> IESIIKTATDTVKSEINAELGVVPSLNAVETGATSNTEPEEAIQTRTVINQHGVSETLVENFLSRAALVSKRSFEYKDHTSSAAQTDKNFFKWTINTRSFVQLRRKLELFTYLRFDAEITILTTVAVNGSSNNTYMGLPNLTLQAMFVPTGALTPEKQDSFHWQSGSNASVFFKISDPPARMTIPFMCINSAYSVFYDGFAGFEKSGLYGINPADTIGNLCVRIVNEHQPVGFTVTVRVYMKPKHIKAWAPRPPRTLPYMSIANANYKGKKRAPNALNAIIGNRDSVKTMPHNIVTT;> GVPTYLLPGSGQFLTTDDHSSAPVLPCFNPTPEMHIPGQVRNMLEVVQVESMMEINNTESAVGMERLKVDISALTDVDQLLFNIPLDIQLDGPLRNTLVGNISRYYTHWSGSLEMTFMFCGSFMATGKLILCYTPPGGSCPTTRETAMLGTHIVWDFGLQSSVTLIIPWISGSHYRMFNNDAKSTNANVGYVTCFMQTNLIVPSESSDTCSLIGFIAAKDDFSLRLMRDSPDIGQIDHLHAAEAAYQ;> SPSAEACGYSDRVLQLKLGNSAIVTQEAANYCCAYGEWPNYLPDHEAVAIDKPTQPETATDRFYTLKSVKWEAGSTGWWWKLPDALNNIGMFGQNVQHHYLYRSGFLIHVQCNATRFHQGALLVVAIPEHQRGAHNTNTSPGFDDIMKGEEGGTFNHPYVLDDGTSLACATIFPHQWINLRTNNSATIVLPWMNAAPMDF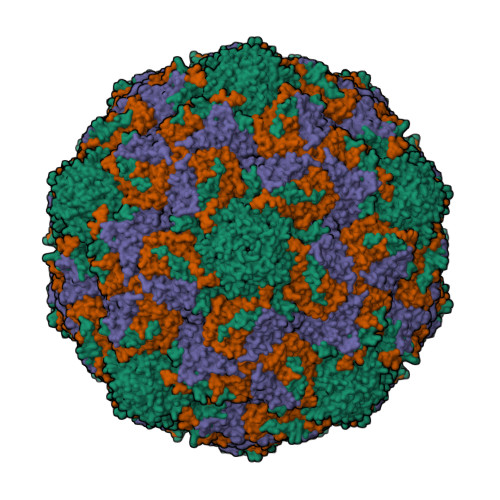PLRHNQWTLAIIPVVPLGTRTMSSMVPITVSIAPMCCEFNGLRHAITQ> SNAMNMLKILRQITQEVNAAPNLEQALKLVVVRLCEALPADACSLFICDDVHGEYVLMATQGLNSKQVGKLRLKFGEGLIGLVGEREEPINLADA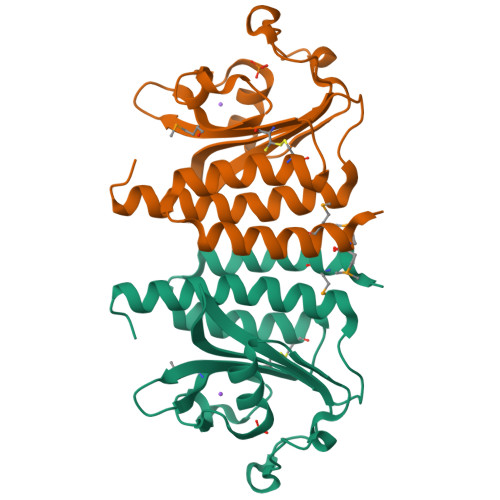PLHPAYKHRPELGEEDYHGFLGIPIIEQGELLGILVIQQLESHHFAEEEEAFCVTLAIHLAAEIAHARAKGALEKL> LMYYESLTKQYPVSKTIRNELIPIGKTLDNIRQNNILESDVKRKQNYEHVKGILDEYHKQLINEALDNCTLPSLKIAAEIYLKNQKEVSDREDFNKTQDLLRKEVVEKLKAHENFTKIGKKDILDLLEKLPSISEDDYNALESFRNFYTYFTSYNKVRENLYSDKEKSSTVAYRLINENFPKFLDNVKSYRFVKTAGILADGLGEEEQDSLFIVETFNKTLTQDGIDTYNSQVGKINSSINLYNQKNQKANGFRKIPKMKMLYKQILSDREESFIDEFQSDEVLIDNVESYGSVLIESLKSSKVSAFFDALRESKGKNVYVKNDLAKTAMSNIVFENWRTFDDLLNQEYDLANENKKKDDKYFEKRQKELKKNKSYSLEHLCNLSEDSCNLIENYIHQISDDIENIIINNETFLRIVINEHDRSRKLAKNRKAVKAIKDFLDSIKVLERELKLINSSGQELEKDLIVYSAHEELLVELKQVDSLYNMTRNYLTKKPFSTEKVKLNFNRSTLLNGWDRNKETDNLGVLLLKDGKYYLGIMNTSANKAFVNPPVAKTEKVFKKVDYKLLPVPNQMLPKVFFAKSNIDFYNPSSEIYSNYKKGTHKKGNMFSLEDCHNLIDFFKESISKHEDWSKFGFKFSDTASYNDISEFYREVEKQGYKLTYTD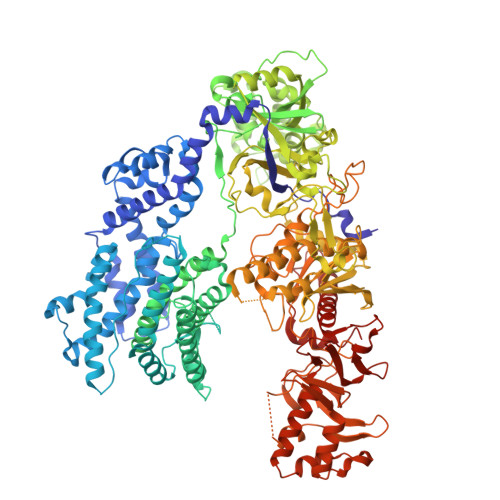IDETYINDLIERNELYLFQIYNKDFSMYSKGKLNLHTLYFMMLFDQRNIDDVVYKLNGEAEVFYRPASISEDELIIHKAGEEIKNKNPNRARTKETSTFSYDIVKDKRYSKDKFTLHIPITMNFGVDEVKRFNDAVNSAIRIDENVNVIGIDRGERNLLYVVVIDSKGNILEQISLNSIINKEYDIETDYHALLDEREGGRDKARKDWNTVENIRDLKAGYLSQVVNVVAKLVLKYNAIICLEDLNFGFKRGRQKVEKQVYQKFEKMLIDKLNYLVIDKSREQTSPKELGGALNALQLTSKFKSFKELGKQSGVIYYVPAYLTSKIDPTTGFANLFYMKCENVEKSKRFFDGFDFIRFNALENVFEFGFDYRSFTQRACGINSKWTVCTNGERIIKYRNPDKNNMFDEKVVVVTDEMKNLFEQYKIPYEDGRNVKDMIISNEEAEFYRRLYRLLQQTLQMRNSTSDGTRDYIISPVKNKREAYFNSELSDGSVPKDADANGAYNIARKGLWVLEQIRQKSEGEKINLAMTNAEWLEYAQTHLL> MIVKRPVSASLARAFFYIVLLSILSTGIALLTLASSLRDAEAINIAGSLKMQSYRLGYDLQSGSPQLNAHRQLFQQALHSPVLTNLNVWYVPEAVKTRYAHLNANWLEMNN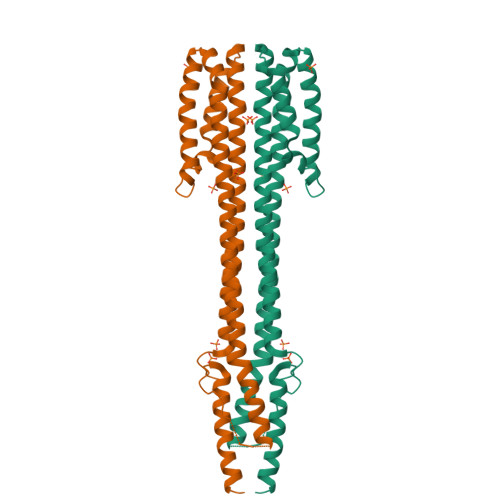RLSKGDLPWYQANINNYVNQIDLFVLALQHYAERKMLLVVAISLAGGIGIFTLVFFTLRRIRHQVVAPLNQLVTASQRIEHGQFDSPPLDTNLPNELGLLAKTFNQMSSELHKLYRSLEHHHHHH>[2x]MGSDKIHHHHHHENLYFQGLLPKYNILTEDQVQKIHENTMKILEEIGIEFEYEPALEVFRREGQKVEGKRVYLTREFVESKLKSAPAEFTLHARNPENNVVIGGDNIVFMPGYGAPFIYELDGSRRKTTLQDYENFAKLAGASKNMHLSGGTMAEPQDIPDGVRHLQMLYSSIKNSDKCFMGSAEGKERAEDSVEIAAILFGGKD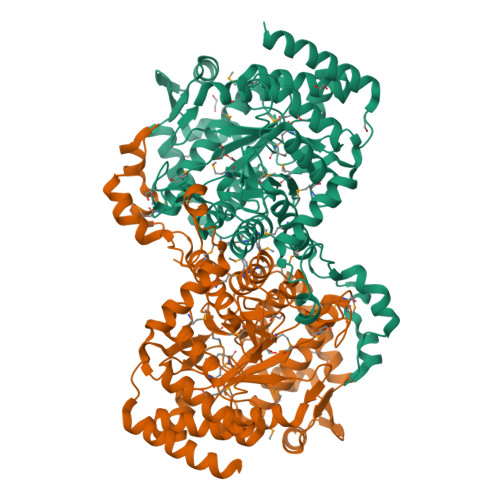VIKEKPVLVSLINSLTPLKYDERMLGALMAYAEAGQAVIIASLVMAGSTGPASLAGTLSLQNAEVLAGISLAQSINPGTPVIYGSTSALSDMRSGSLSIGSPECALFISASAQLARFYGVPSRSGGGLNDSKTVDAQAGYESMMTLMAANLTGVNFVLHTAGILQYFMAMSYEKFIMDDEIAGMLLHYMKGYTFDEDGMAFDVIEKVGPGGHFLTQKHTRKNHKREFYTPTLSDRSAYDTWAKEKLETKQRAHARWQQILANYVPPALDPEIDAKLQAFIAQRGKEVGEE> GPGSRPKNMTPYRSPP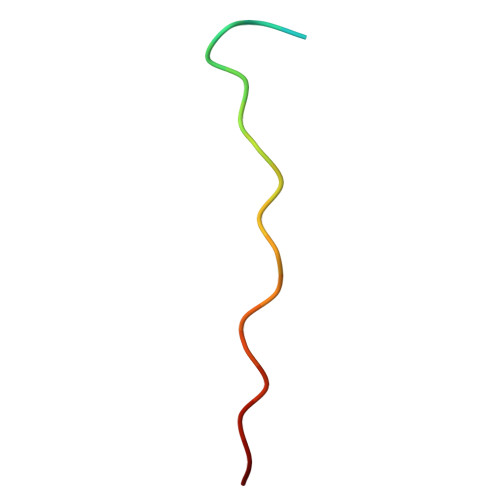PYVPP>MNKLVGLLVSSLFLASILIGIAPAITTTALTPPVSAGGIQAYLLTGSGAPASGLVLFVVNVSNIQVSSSNVTNVISTVVSNIQINAKTENAQTGATTGSVTVRFPTSGYNAYYDSVDKVVFVVVSFLYPYTTTSVNIPLSYLSKYLPGLLTAQPYDETGAQVTSVSSTPFGSLIDTSTGQQILGTNPVLTSYNSYTTQANTNMQEGVVSGTLTSFTLGGQSFSGSTVPVILYAPFIFSNSPYQAGLYNPMQVNGNLGSLSSEAYYHPVIWGRALINTTLIDTYASGSVPFTFQLNYSVPGPLTINMAQLAWIASINNLPTSFTYLSYKFSNGYESFLGIISNSTQLTAGALTINPSGNFTINGKKFYVYLLVVGSTNSTTPVEYVTKLVVEYPSSTNFLPQGVTVTTSSNKYTLPVYEIGGPAGTTITLTGNWYSTPYTVQITVGSTPTLTNYVSQILLKAVAYEGINVSTTQSPYYSTAILSTPPSEISITGSSTITAQGKLTATSASATVNLLTNATLTYENIPLTQYSFNGIIVTPGYAAINGTTAMAYVIGALYNKTSDYVLSFAGSQEPMQVMNNNLTEVTTLAPFGLTLLAPSVPATETGTSPLQLEFFTVPSTSYIALVDFGLWGNLTSVTVSAYDTVNNKLSVNLGYFYGIVIPPSISTAPYNYQNFICPNNYVTVTIYDPDAVLDPYPSGSFTTSSLPLKYGNMNITGAVIFPGSSVYNPSGVFGYSNFNKGAAVTTFTYTAQSGPFSPVALTGNTNYLSQYADNNPTDNYYFIQTVNGMPVLMGGLSIVASPVSASLPSSTSSPGFMYLLPSAAQVPSPLPGMATPNYNLNIYITYKIDGATVGNNMINGLYVASQNTLIYVVPNGSFVGSNIKLTYTTTDYAVLHYFYSTGQYKVFKTVSVPNVTANLYFPSSTTPLYQLSVPLYLSEPYYGSPLPTYIGLGTNGTSLWNSPNYVLFGVSAVQQYLGFIKSISVTLSNGTTVVIPLTTSNMQTLFPQLVGQELQACNGTFQFGISITGLEKLLNLNVQQLNNSILSVTYHDYVTGETLTATTKLVALSTLSLVAKGAGVVEFLLTAYPYTGNITFAPPWFIAENVVKQPFMTYSDLQFAKTNPSAILSLSTVNITVVGLGGKASVYYNSTSGQTVITNIYGQTVATLSGNVLPTLTELAAGNGTFTGSLQFTIVPNNTVVQIPSSLTKTSFAVYTNGSLAIVLNGKAYSLGPAGLFLLPFVTYTGSAIGANATAIITVS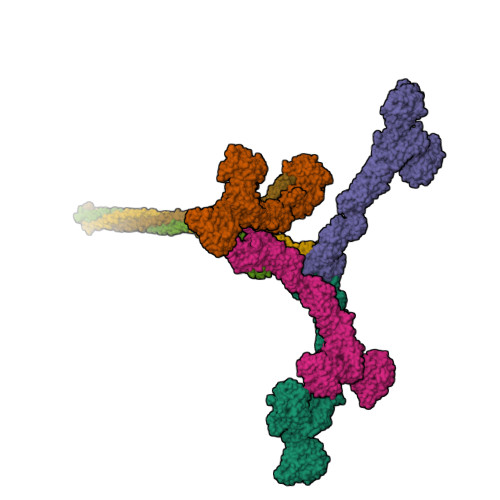DGVGTSTTQVPITAENFTPIRLAPFQVPAQVPLPNAPKLKYEYNGSIVITPQQQVLKIYVTSILPYPQEFQIQAFVYEASQFNVHTGSPTAAPVYFSYSAVRAYPALGIGTSVPNLLVYVQLQGISNLPAGKYVIVLSAVPFAGGPVLSEYPAQLIFTNVTLTQ[4x];>MNKNLAILTPIVLLSLVLAPIAISAVTINGITFYSPVPNQTYKYGQQLVLSIQSQPNALVTLYVYDPKGNVVYNNVYQTNSSGGLTATIATFGSTPGFTTVGTYTVSLSVQGTTSESASVNVQYVPLTSTITATVVNQEGSPLAGATVQLYNTTSGSNTLVATQTTNSQGVATFTVLSFPGVTQTFKLVASLQGYAASTASVSITGQQNASVTITLVPAVVTIAPMYVIQNGTVIGSGPSLSSIVVYQGLPAYILAQVSFAGQRVTTAPVSAQVYYPNGTQTVKASVITSGKYAGMYNITIMPPTESVQNYVFQLLIVANYTTSSGQTLSTKYLMSVQANQNLQALVNKEISSLVQNITNLEKTVNNLQTQISTLNSSLSSLSQRITSLQNTLASLNSTISSLSGTASSLSSQLNALQGKISSLNSSITNLSGQLNSLQSKVNSLTPLVYGGIIAGIIGLIVAIVAIVLVYRKIS[3x]3-[(4-methoxyphenyl)methyl]-5-oxidanyl-~{N}-[3-(trifluoromethyl)phenyl]-1,2,3-triazole-4-carboxamide | C18 H15 F3 N4 O3 | 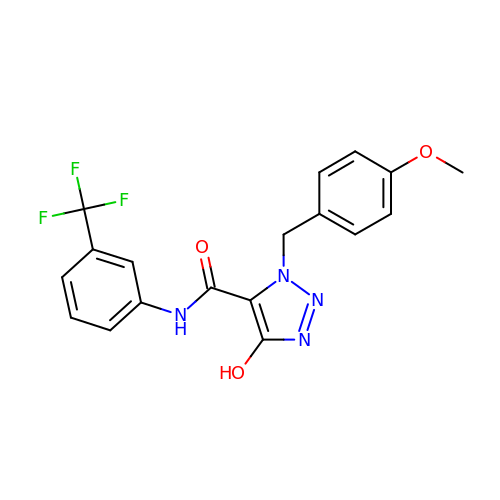IMCLZLUHJZCWCW-UHFFFAOYSA-N> PTALERVQKEGVLRVITRNSPATYFQDRNGETGFEYELAKRFAERLGVELKIETADNLDDLYAQLSREGGPALAAAGLTPGREDDASVRYSHTYLDVTPQIIYRNGQQRPTRPEDLVGKRIMVLKGSSHAEQLAELKKQYPELKYEESDAVEVVDLLRMVDVGDIDLTLVDSNELAMNQVYFPNVRVAFDFGEARGLAWALPGGDDDSLMNEVNAFLDQAKKEGLLQRLKDRYYGHVDVLGYVGAYTFAQHLQQRLPRYESHFKQSGKQLDTDWRLLAAIGYQESLWQPGATSKTGVRGLMMLTNRTAQAMGVSNRLDPKQSIQGGSKYFVQIRSELPESIKEPDRSWFALAAYNIGGAHLEDARKMAEKEGLNPNKWLDVKKMLP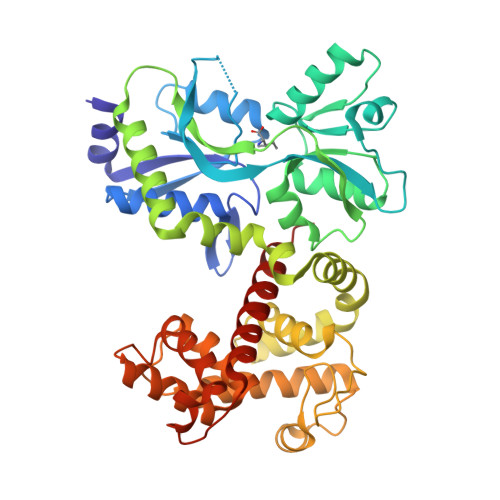RLAQKQWYAKTRYGYARGGETVHFVQNVRRYYDILTWVTQPQ In the eukaryotic cytoplasm, Get3 delivers tail-anchored (TA) integral membrane proteins, defined by a single transmembrane helix at their C terminus, to the endoplasmic reticulum. Get3d is conserved across land plants and photosynthetic bacteria and includes a distinctive C-terminal α-crystallin domain. Distinct features of Get3d include an incomplete active site, a “closed” conformation in the apo-state, and a hydrophobic chamber. Both homologs have ATPase activity and are capable of binding TA proteins, supporting a potential role in TA protein targeting.

We generated a construct without the chloroplast transit peptide (Δ1–57) that purified as a single peak via size-exclusion chromatography, consistent with a homodimer. While the sequence suggested missing residues for ATP binding, only crystals grown in the presence of ADP resulted in diffraction. Final crystals, grown by sitting drop in 50 mM sodium cacodylate (pH 5.47), 50 mM lithium sulfate, and 30% PEG-4000, were frozen with the addition of 30% glycerol as a cryoprotectant, and a complete native dataset was collected to 2.0 Å resolution in the space group P 1 21 1. No density for nucleotide was visible in the putative active site; however, there was clear density for an inorganic phosphate and an Mg2+ ion. Like structures of Get3 homologs, AtGet3d is a homodimer with a core nucleotide-binding domain and an α-helical client-binding domain (CBD). A structural alignment suggests that, after NosGet3d, AtGet3d is most similar to the closed conformation of yeast Get3 (45). As opposed to the groove seen in fungal Get3 structures, the CBD of AtGet3d is a chamber. Considering these results, the density, and the properties of the binding site, a phosphatidic acid was built into this density. The aliphatic chains fit the two tubes of density, whereas the phosphate head group forms a salt bridge with R176, R182, and a possible H-bond with Q136. First, in AtGet3d, a salt bridge formed between K107 in the Get3 domain to E404 in the αCD of the opposite monomer is reminiscent of a salt bridge between the homologous yeast Get3 K69 to D74 of Get4.

>[2x]MTKFVTFLGKGGSGKTTAAVFAAQHYALAGLSTCLVIHNQDPSAEFLLGSKIGTSPTLINDNLSVIRLETTKMLLEPLKQLKQADARLNMTQGVLEGVVGEELGVLPGMDSIFSMLELERLVGFFRQATRKNHKGKPFDVIIYDGISTEETLRMIGLSSKTRLYAKYLRSLAEKTDLGRLTSPSIMRFVDESMNINSNKSPFDGMTSPAMWDTLERFLETGASAWRDPERFRSFLVMDPNNPMSVKAALRYWGCTVQAGSHVSGAFAISSSHLTSQIPKADFVPLPFASASVPFTITGLDWDKILLDQANSSIRELLSETVSHGTSLTQTVMFDTAKKLVTLFMPGFEKSEIKLYQYRGGSELLIEAGDQRRVIHLPSQIQGKVGGAKFVDRSLIVTMRLEHHHHHH>NELWFIDAQAMFQNYANLRSFSKSNANEINTTIGGFVFGRKARKQVIHVLFAYAEDLTESNRQFLESSLSADIELVGNLNIDGQSQILPGGQFTLQLTSRMLENRSISEFLDMNVMFNNEHVLMEGASCVSRVGYEWSLRAGREQEDVKSAAERLSMASFRFTYLNAEHGLVIREQKPEAAQQKYLDKFSKGAVPYKDVIEFTAMQSLTRDTSNDTEDQKLVPTVKVTKDNKHFTRLVTIGEVVFPAFFGDSSLDLYKRSREAFNRRANNTMMVTVNGIRAGRGVTTTTSATYLPPGWVSLLHLQLPTKWTDNEQRNYRIRLHKLFNLPSSKPVLRLSQALALHSESARLTNKKLIREPHLSITNYQPVGEITTVNGPYNYHHYMQDGIDDSGWGCAYRSFQTIWSWFILNGYTDKPVPSHREIQQALVDIQDKQAKFVGSRQWIGSTEISFVLNELLKLECRFIATNSGAEVVERVRELARHFETSGTPVMIGGNMLAHTILGVDFNDTTGETKFLVLDPHYTGSEDIKTITSKGWCAWKPASFWSKDHFYNMVLPQ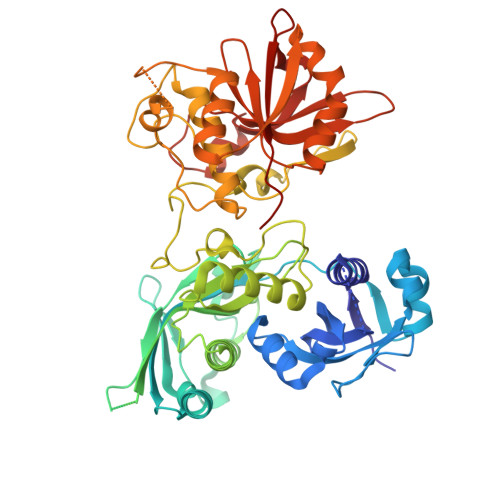PPSDAI[2x]Citrullination, the loss of a positive charge on the arginine side chain to form citrulline, is catalyzed by peptidylarginine deiminase 4 (PAD4) of the PAD enzyme family. PAD4 is implicated in rheumatoid arthritis (RA), where citrullinated epitopes serve as important diagnostic and pathological factors. The active form of PAD4 is a homodimer, and dimerization greatly affects enzyme activity because monomeric mutants are less active. In this study, we identified GAGs as physiological allosteric coactivators of PAD4.

Enzyme activity also depends on calcium ion concentration. A PAD4 monomer has five binding sites for Ca2+, and its saturation results in conformational changes, leading to maturation of the active site (14–16). The calcium-binding sites remained unresolved, even in our 10 mM CaCl2 structure of PAD4.

>[2x]MGHHHHHHHHHHHMAQGTLIRVTPEQPTHAVCVLGTLTQLDICSSAPEDCTSFSINASPGVVVDIAHGPPAKKKSTGSSTWPLDPGVEVTLTMKVASGSTGDQKVQISYYGPKTPPVKALLYLTGVEISLCADITRTGKVKPTRAVKDQRTWTWGPCGQGAILLVNCDRDNLESSAMDCEDDEVLDSEDLQDMSLMTLSTKTPKDFFTNHTLVLHVARSEMDKVRVFQATRGKLSSKCSVVLGPKWPSHYLMVPGGKHNMDFYVEALAFPDTDFPGLITLTISLLDTSNLELPEAVVFQDSVVFRVAPWIMTPNTQPPQEVYACSIFENEDFLKSVTTLAMKAKCKLTICPEEENMDDQWMQDEMEIGYIQAPHKTLPVVFDSPRNRGLKEFPIKRVMGPDFGYVTRGPQTGGISGLDSFGNLEVSPPVTVRGKEYPLGRILFGDSCYPSNDSRQMHQALQDFLSAQQVQAPVKLYSDWLSVGHVDEFLSFVPAPDRKGFRLLLASPRSCYKLFQEQQNEGHGEALLFEGIKKKKQQKIKNILSNKTLREHNSFVERCIDWNRELLKRELGLAESDIIDIPQLFKLKEFSKAEAFFPNMVNMLVLGKHLGIPKPFGPVINGRCCLEEKVCSLLEPLGLQCTFINDFFTYHIRHGEVHCGTNVRRKPFSFKWWNMVP> GSHMRKKIFKPEELRQALMPTLE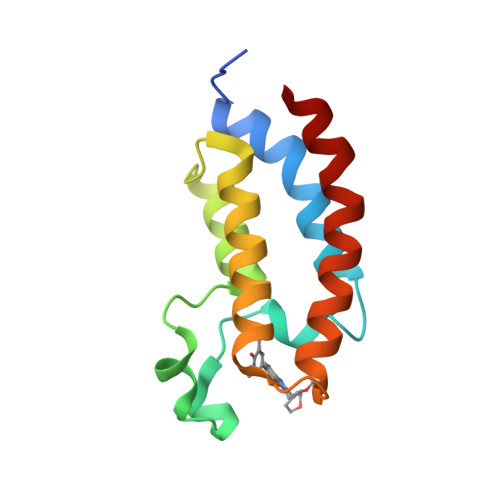ALYRQDPESLPFRQPVDPQLLGIPDYFDIVKNPMDLSTIKRKLDTGQYQEPWQYVDDVWLMFNNAWLYNRKTSRVYKFCSKLAEVFEQEIDPVMQSLG> GSERRAVYIGALFPMSGGWPGGQACQPAVEMALEDVNSRRDILPDYELKLIHHDSKCDPGQATKYLYELLYNDPIKIILMPGCSSVSTLVAEAARMWNLIVLSYGSSSPALSNRQRFPTFFRTHPSATLHNPTRVKLFEKWGWKKIATIQQTTEVFTSTLDDLEERVKEAGIEITFRQSFFSDPAVPVKNLKRQDARIIVGLFYETEARKVFCEVYKERLFGKKYVWFLIGWYADNWFKIYDPSINCTVDEMTEAVEGHITTEIVMLNPANTRSISNMTSQEFVEKLTKRLKRHPEETGGFQEAPLAYDAIWALALALNKTSGGGGRSGVRLEDFNYNNQTITDQIYRAMNSSSFEGVSGHVVFDASGSRMAWTLIEQLQGGSYKKIGYYDSTKDDLSWSKTDKWIGGSPPADQTLVIKTFRFLSQKLFISVSVLSSLGIVLAVVCLSFNIYNSHVRYIQNSQPNLNNLTAVGCSLALAAVFPLGLDGYHIGRNQFPFVCQARLWLLGLGFSLGYGSMFTKIWWVHTVFTKKEEKKEWRKTLEPWKLYATVGLLVGMDVLTLAIWQIVDPLHRTIETFAKEEPKEDIDVSILPQLEHCSSRKMNTWLGIFYGYKGLLLLLGIFLAYETKSVSTEKINDHRAVGMAIYNVAVLCLITAPVTMILSSQQDAAFAFASLAIVFSSYITLVVLFVPKMRRLITRGEWQSEAQDTMKTGSSTNNNEEEKSRLLEKENRELEKIIAEKEERVSELRHQLQSRLEVLFQ;> GWARGAPRPPPSSPPLSIMGLMPLTKEVAKGSIGRGVLPAVELAIEQIRNESLLRPYFLDLRLYDTECDNAKGLKAFYDAIKYGPNHLMVFGGVCPSVTSIIAESLQGWNLVQLSFAATTPVLADKKKYPYFFRTVPSDNAVNPAILKLLKHYQWKRVGTLTQDVQRFSEVRNDLTGVLYGEDIEISDTESFSNDPCTSVKKLKGNDVRIILGQFDQNMAAKVFCCAYEENMYGSKYQWIIPGWYEPSWWEQVHTEANSSRCLRKNLLAAMEGYIGVDFEPLSSKQIKTISGKTPQQYEREYNNKRSGVGPSKFHGYAYDGIWVIAKTLQRAMETLHASSRHQRIQDFNYTDHTLGRIILNAMNETNFFGVTGQVVFRNGERMGTIKFTQFQDSREVKVGEYNAVADTLEIINDTIRFQGSEPPKDKTIILEQLRKISLPLYSILSALTILGMIMASAFLFFNIKNRNQKLIKMSSPYMNNLIILGGMLSYASIFLFGLDGSFVSEKTFETLCTVRTWILTVGYTTAFGAMFAKTWRVHAIFKNVKMKKKIIKDQKLLVIVGGMLLIDLCILICWQAVDPLRRTVEKYSMEPDPAGRDISIRPLLEHCENTHMTIWLGIVYAYKGLLMLFGCFLAWETRNVSIPALNDSKYIGMSVYNVGIMCIIGAAVSFLTRDQPNVQFCIVALVIIFCSTITLCLVFVPKLITLRTNPDAATQNRRFQFTQN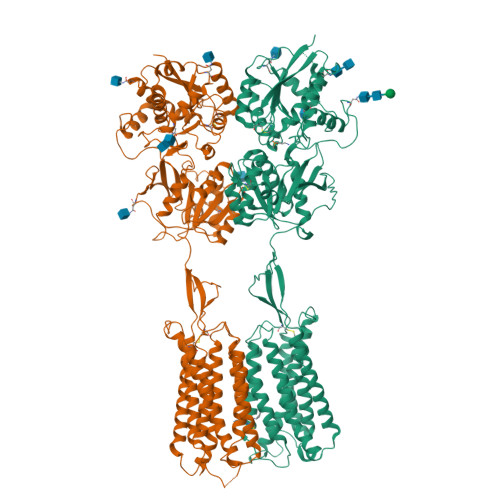QKKEDSKTSTSVTSVNQASTSRLEGLQSENHRLRMKITELDKDLEEVTMQLQDT2,4-diamino-6-{[(S)-[5-chloro-8-fluoro-4-oxo-3-(pyridin-3-yl)-3,4-dihydroquinazolin-2-yl](cyclopropyl)methyl]amino}pyrimidine-5-carbonitrile 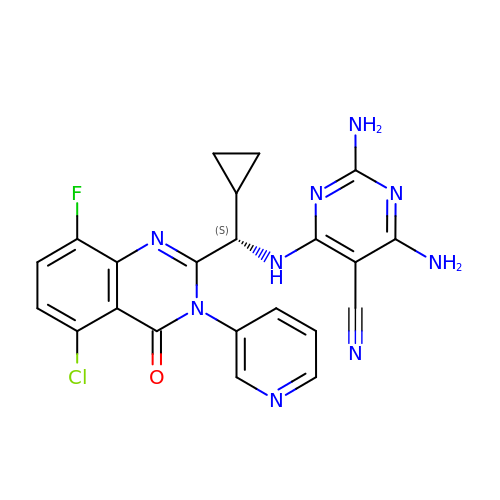| C22 H17 Cl F N9 O | XDSXYMOZKDUASY-INIZCTEOSA-N>SNAMKIVIAPDSYKESLSALEVATAIEQGFREIWPDADYLKLPLADGGEGTVEAMVEATAGRIVHVEVTGPLGHRVNAFYGLSGDARSAFIEMAAASGLEQVPPAQRDPLKTTSWGTGELIRHALDAGVEHIIIGIGGSATNDGGAGMVQALGARLRDAQGNDIAQGGIGLETLASIDISGLDKRLSACHIEVACDVTNPLTGKEGASAVFGPQKGATPEMIERLDTALTRYAHLIARDLHVDVLDLAGGGAAGGMGAALYAFCGAQLRRGIEIVTDALHLEACLADADLVITGEGRIDSQTIHGKVPIGVANIAKRYNKPVIGIAGSLTADVSVVHEHGLDAVFSV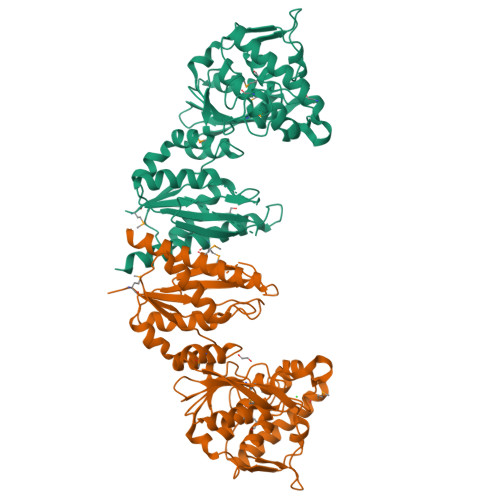IYTICTLEDALKNASENVRMTARNVAATLKAGQQLR[2x]>MNQNLLVTKRDGSTERINLDKIHRVLDWAAEGLHNVSISQVELRSHIQFYDGIKTSDIHETIIKAAADLISRDAPDYQYLAARLAIFHLRKKAYGQFEPPALYDHVVKMVEMGKYDNHLLEDYTEEEFKQMDTFIDHDRDMTFSYAAVKQLEGKYLVQNRVTGEIYESAQFLYILVAACLFSNYPRETRLQYVKRFYDAVSTFKISLPTPIMSGVRTPTRQFSSCVLIECGDSLDSINATSSAIVKYVSQRAGIGINAGRIRALGSPIRGGEAFHTGCIPFYKHFQTAVKSCSQGGVRGGAATLFYPMWHLEVESLLVLKNNRGVEGNRVRHMDYGVQINKLMYTRLLKGEDITLFSPSDVPGLYDAFFADQEEFERLYTKYEKDDSIRKQRVKAVELFSLMMQERASTGRIYIQNVDHCNTHSPFDPAIAPVRQSNLCLEIALPTKPLNDVNDENGEIALCTLSAFNLGAINNLDELEELAILAVRALDALLDYQDYPIPAAKRGAMGRRTLGIGVINFAYYLAKHGKRYSDGSANNLTHKTFEAIQYYLLKASNELAKEQGACPWFNETTYAKGILPIDTYKKDLDTIANEPLHYDWEALRESIKTHGLRNSTLSALMPSETSSQISNATNGIEPPRGYVSIKASKDGILRQVVPDYEHLHDAYELLWEMPGNDGYLQLVGIMQKFIDQSISANTNYDPSRFPSGKVPMQQLLKDLLTAYKFGVKTLYYQNTRDGAEDAQDDLVPSIQDDGCESGACKI[4x];>[4x]AYTTFSQTKNDQLKEPMFFGQPVNVARYDQQKYDIFEKLIEKQLSFFWRPEEVDVSRDRIDYQALPEHEKHIFISNLKYQTLLDSIQGRSPNVALLPLISIPELETWVETWAFSETIHSRSYTHIIRNIVNDPSVVFDDIVTNEQIQKRAEGISSYYDELIEMTSYWHLLGEGTHTVNGKTVTVSLRELKKKLYLCLMSVNALEAIRFYVSFACSFAFAERELMEGNAKIIRLIARDEALHLTGTQHMLNLLRSGADDPEMAEIAEECKQECYDLFVQAAQQEKDWADYLFRDGSMIGLNKDILCQYVEYITNIRMQAVGLDLPFQ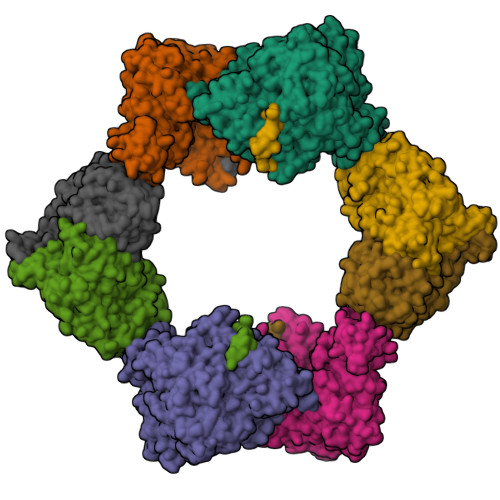TRSNPIPWINTWLVSDNVQVAPQEVEVSSYLVGQIDSEVDTDDLSNFQL>[4x]GPGSMVSHPEQSRHLATAIPGP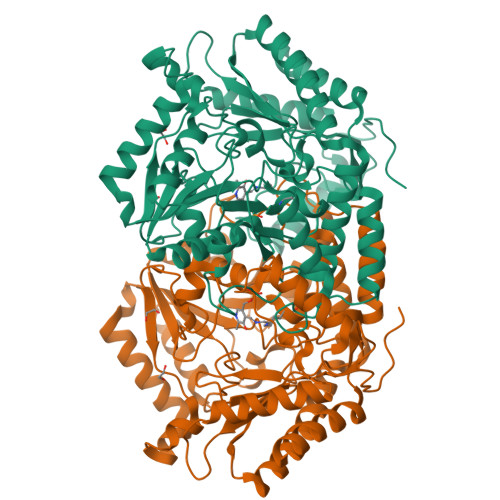RSQALIDRKGTAVARGVGTTMPVYAVRAGGGIVEDVDGNRLIDLGSGIAVTTVGNSAPKVVEAVRSQVGDFTHTCFMVTPYEGYVAVCEQLNRLTPVRGDKRSALFNSGSEAVENAVKIARSHTHKPAVVAFDHAYHGRTNLTMALTAKVMPYKDGFGPFAPEIYRAPLSYPFRDAEFGKELATDGELAAKRAITVIDKQIGADNLAAVVIEPIQGEGGFIVPADGFLPTLLDWCRKNDVVFIADEVQTGFARTGAMFACEHEGIDPDLIVTAKGIAGGLPLSAVTGRAEIMDSPHVSGLGGTYGGNPIACAAALATIETIESEGLVARAQQIEKIMKDRLGRLQAEDDRIGDVRGRGAMIAMELVKAGTTEPDADLTKALCAGAHAAGVIVLSCGTYGNVVRFLPPLSIGDDLLNEGLDVLEEVLRGA> KNYSVLYFQQKVDHFGFNTVKTFNQRYLVADKYWKKNGGSILFYTGNEGDIIWFCNNTGFMWDVAEELKAMLVFA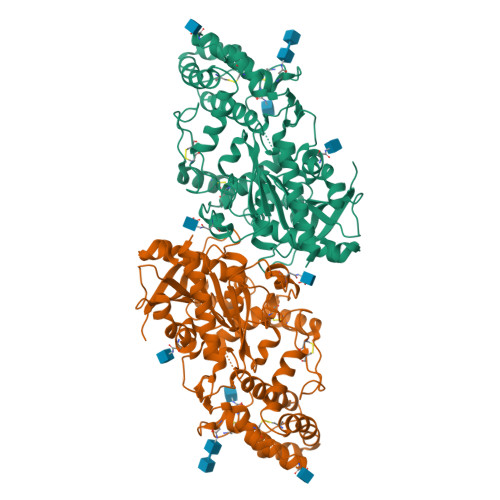EHRYYGESLPFGDNSFKDSRHLNFLTSEQALADFAELIKHLKRTIPGAENQPVIAIGGSYGGMLAAWFRMKYPHMVVGALAASAPIWQFEDLVPCGVFMKIVTTDFRKSGPHCSESIHRSWDAINRLSNTGSGLQWLTGALHLCSPLTSQDIQHLKDWISETWVNLAMVDYPYASNFLQPLPAWPIKVVCQYLKNPNVSDSLLLQNIFQALNVYYNYSGQVKCLNISETATSSLGTLGWSYQACTEVVMPFCTNGVDDMFEPHSWNLKELSDDCFQQWGVRPRPSWITTMYGGKNISSHTNIVFSNGELDPWSGGGVTKDITDTLVAVTISEGAHHLDLRTKNALDPMSVLLARSLEVRHMKNWIRDFYDS> GGGKATGTNEQSEKVVVNVPQFDADSAYLYVKNQVDFGPRVPNTKEHVACGNYLAGKLEAFGAKVTNQYADLIAYDGTLLKARNIIGSYKPESKKRIALFAHWDTRPWADNDADEKNHHTPILGANDGASGVGALLEIARLVNQQQPELGIDIIFLDAEDYGTPQ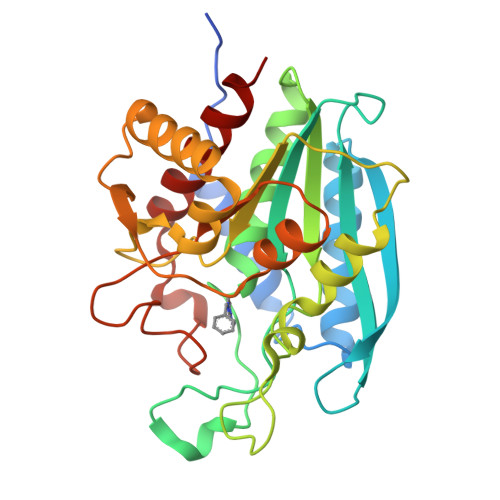FYEGKHKEEAWCLGSQYWSRNPHVQGYNARFGILLDMVGGENSVFLKEGYSEEFAPDINKKVWKAAKKAGYGKTFIDERGDTITDDHLFINRLARIKTIDIIPNDPETGFPPTWHTIHDNMDHIDKNTLKAVGQTVLEVIYNEK> VAQGPNGRALAESMNPDLLSAIQQHISIERY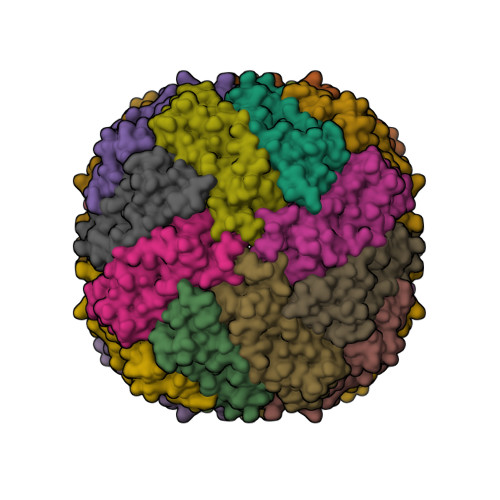ASVTFLAMSIWCAERELAGFYQFFDGEAKDEQSHAVHFTQYLIARSQSNDLQTLDAPRQNWDSLASLMATAFQMEADTTSSIQSVYALAERNSDTRTTVFLDPLIEAQIQSEDQFAYLLGRVKFANGDPTALLVIDNELRAGQTQRG>PPPLSHCGRAAPCEPLRYNVCLGSVLPYGATSTLLAGDSDSQEEAHGKLVLWSGLRNAPRCWAVIQPLLCAVYMPKCENDRVELPSRTLCQATRGPCAIVERERGWPDFLRCTPDRFPEGCTNEVQNIKFNSSGQCEVPLVRTDNPKSWYEDVEGCGIQCQNPLFTEAEHQDMHSYIAAFGAVTGLCTLFTLATFVADWRNSNRYPAVILFYVNACFFVGSIGWLAQFMDGARREIVCRADGTMRLGEPTSNETLSCVIIFVIVYYALMAGVVWFVVLTYAWHTSFKALGTTYQPLSGKTSYFHLLTWSLPFVLTVAILAVAQVDGDSVSGICFVGYKNYRYRAGFVLAPIGLVLIVGGYFLIRGVMTLFSIKSNHAKALIVYGSTTGNTEYTAETIARELADAGYEVDSRDAASVEAGGLFEGFDLVLLGCSTWGDDSIELQDDFIPLFDSLEETGAQGRKVACFGCGDSSWEYFCGAVDAIEEKLKNLGAEIVQDGLRIDGDPRAARDDIVGWAHDVRGAIKINETMLRLGIFGFLAFGFVLITFSCHFYDFFNQAEWERSFRDYVLCQANVTIGLPTKQPIPDCEIKNRPSLLVEKINLFAMFGTGIAMSTWVWTKATLLIWRRTWCRLTGQSDDHHHHHHHHHH[2x]

The smoothened receptor (SMO), a Class Frizzled seven-transmembrane helices (7TM) G protein-coupled receptor (GPCR), is a key component in this signalling pathway. The activity of SMO is suppressed by the PTCH receptor, a 12TM protein. This suppression is disabled when Hh binds to PTCH, leading to phosphorylation of SMO's cytoplasmic region5, which induces the translocation of GLI transcription factors into the nucleus to activate target genes. Here, we present the crystal structure of the multi-domain human SMO in complex with a specially designed TMD ligand, shedding light on interactions between the CRD and TMD.

To facilitate crystallization, human SMO was engineered by fusion of a Flavodoxin (FLA)16 protein between helices V and VI, replacing part of intracellular loop 3 (ICL3) between P434 and S443. The resulting SMO–FLA construct was co-expressed with vismodegib, and then purified and crystallized in complex with TC114 using the lipidic cubic phase method. We determined the structure using room temperature data collected at an X-ray free-electron laser (XFEL) source at 2.9 Å resolution. At the same time, we also solved the structure with data from 12 cryo-cooled crystals collected at a synchrotron source at 3.0 Å resolution. Since the room temperature XFEL crystal structure potentially represents a closer-to-native receptor conformation and at a slightly higher resolution than the synchrotron structure obtained at cryo-cooled conditions, we describe the XFEL SMO structure below, unless noted otherwise. One of these ligands, TC114, with the 4-nitro group substitution, was predicted to form an electrostatic interaction with the protonated ɛ-amine of K395. Analysis of our multi-domain SMO structures indicated that the nitro group introduced in the TC114 ligand does interact strongly with K395 in SMO as designed, and enhance the π–π stacking between the benzoyl group and F484 on helix VI. Therefore, we conclude that TC114 stabilizes the multi-domain SMO by keeping helix VI in a stable conformation that in turn enhances the hydrophobic interaction between the extended ECL3 and the CRD hydrophobic groove. The overall SMO structure shares a canonical GPCR 7TM bundle fold with an amphipathic helix VIII running parallel to the membrane plane.> MASMTGGQQMGRGSAGVLPAHGTQHGIRLPLRSGLGGAPLGLRLPRETDEEPEEPGRRGSFVEMVDNLRGKSGQGYYVEMTVGSPPQTLNILVDTGSSNFAVGAAPHPFLHRYYQRQLSSTYRDLRKGVYVP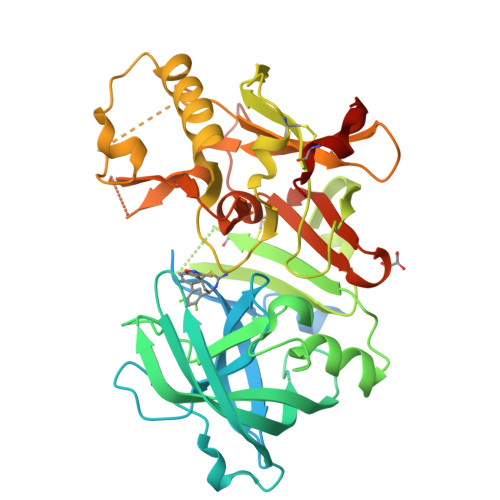YTQGKWEGELGTDLVSIPHGPNVTVRANIAAITESDKFFINGSNWEGILGLAYAEIARPDDSLEPFFDSLVKQTHVPNLFSLQLCGAGFPLNQSEVLASVGGSMIIGGIDHSLYTGSLWYTPIRREWYYEVIIVRVEINGQDLKMDCKEYNYDKSIVDSGTTNLRLPKKVFEAAVKSIKAASSTEKFPDGFWLGEQLVCWQAGTTPWNIFPVISLYLMGEVTNQSFRITILPQQYLRPVEDVATSQDDCYKFAISQSSTGTVMGAVIMEGFYVVFDRARKRIGFAVSACHVHDEFRTAAVEGPFVTLDMEDCGYNIPQTDEST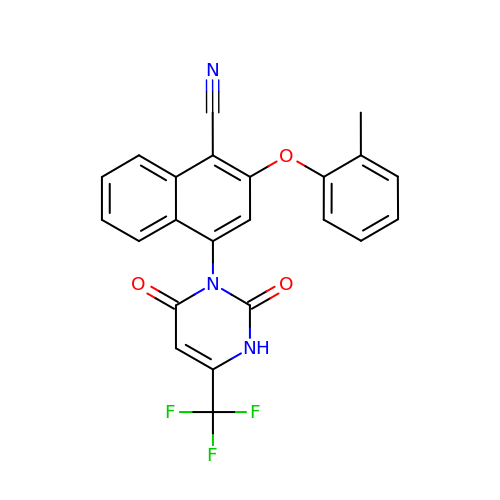4-[2,4-bis(oxidanylidene)-6-(trifluoromethyl)-1H-pyrimidin-3-yl]-2-(2-methylphenoxy)naphthalene-1-carbonitrile | C23 H14 F3 N3 O3 | JBKRLZPXWNTYBD-UHFFFAOYSA-N>[3x]GSQIPASEQETLVRPKPLLLKLLKSVGAQKDTYTMK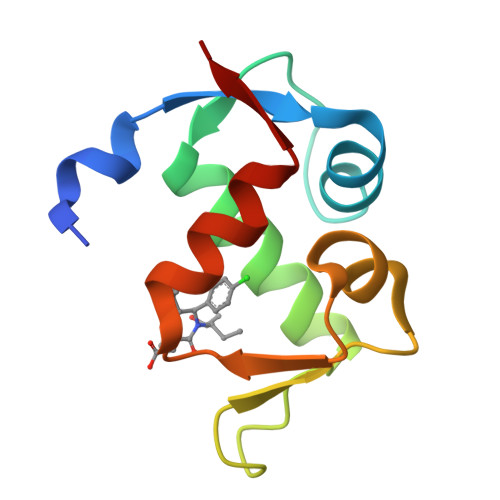EVLFYLGQYIMTKRLYDEKQQHIVYCSNDLLGDLFGVPSFSVKEHRKIYTMIYRNLVVVN>[12x]GMTGKISALDLASGELSEPTKAYFAKCEEKLGLVPNVLKAYAFDDKKLRAFTDIYNDLMLGESGLSKLDREMIAVAVSSINHCYYCL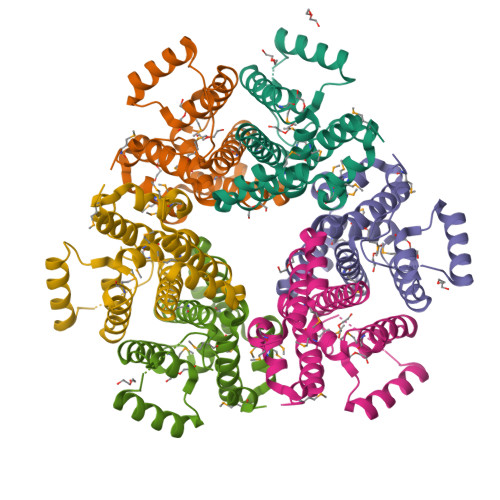TAHGAAVRQLSGDPALGEMLVMNFRAADLSPRQTAMLEFAVKLTEEPAKIVEADRAALRKAGFSDRDIWDIASTAAFFNMSNRVAAAIDMRPNDEYHAMAR> LSPAQVAGSWTFYVQGAEQDACTVTLKKDRTFSAQVSCLQAWLGRTPTTWSPTPDGLLLIGK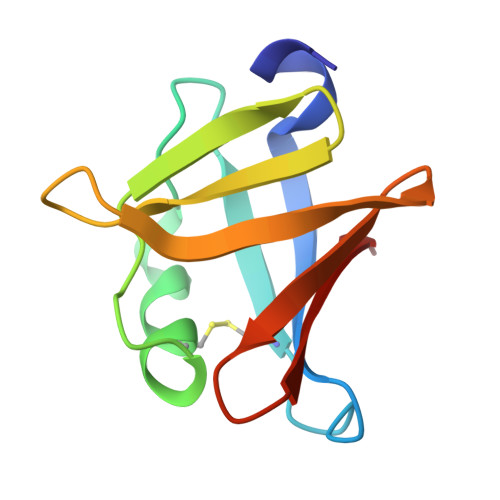DGSQSLFLELREAGRYEGSVEGSKTLVMQRA5-azanyl-3-(1~{H}-indol-6-yl)-1~{H}-pyrazole-4-carbonitrile | C12 H9 N5 | 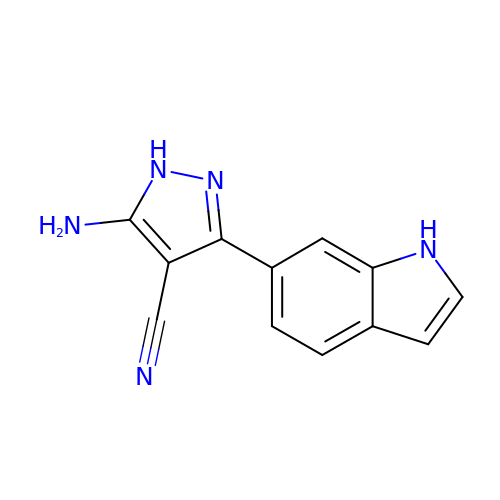ALVYLOVBZSBJDI-UHFFFAOYSA-N>MENDMSSNQTLAEKKIPVSEVPSATLKMLTSQAEGVARPGGIFTKGDLINIKLYVKHSLELPFTLEGVKEYIGYNDIDIDGLKPAKMATLFKEIHDHALSWSGVESKVQQQSIDLENAGKQITLTGDEIISVIDQMPIIERVKNKLGDLTDKQLAEITYTNDDKEIAVELGNILESMKKDIKRQQENTQKVKTAVSDFKLKLIGGELSDGTIAQGLQPQISSKKKLMDDNNLSTTIKDLQSKIDEKNKEIDQFQKDYNKYVGLAFSGMVGGIISWAITGGIFGDKAEKARKQKNKLIDEVKDLQSQVKDKSALQTSVQNLSLSFAGIHTSMVDAEEALNHLDFMWNTMLTQITTSRDKFDDINDALKLTSFVIAFKQVIEPWRDVQGSAAQLIQTFDEALAEYKKLYH[2x]

α-Xenorhabdolysin is a PFT that has been first isolated from the bacterium Xenorhabdus nematophila. Xenorhabdolysins are also found in other entomopathogenic bacteria, such as Photorhabdus luminescens, and human pathogenic bacteria, such as Yersinia enterocolitica and Proteus mirabilis. They are composed of two subunits, namely XaxA (45 kDa) and XaxB (40 kDa) and are only active when the two components act together. Xenorhabdolysins, which were suggested to be binary toxins, perforate the membranes of erythrocytes, insect granulocytes and phagocytes and induce apoptosis. In contrast to previous predictions, XaxAB is therefore not a typical binary toxin, but rather a bi-component α-PFT.

XaxA crystallized in orthorhombic space group P212121 with a unit cell dimension of 67 × 90 × 153 Å and two molecules per asymmetric unit (AU). Phases were determined using the anomalous sulfur signal of the merged datasets and HKL2MAP, the graphical interface for SHELX C/D/E. The obtained phases combined with the given sequence and a few placed α-helices in the density with COOT were sufficient enough for phenix autobuild to almost completely build the structure of XaxA. Interestingly, XaxA contains two large loops connecting the helices, a big hook-shaped loop (lp1, aa 136–169) between helices αB and αC at the top of the tail domain and an additional loop (lp2, aa 202–215) dividing helix αC. In XaxA, the tip of the coiled-coil, predicted as hydrophobic transmembrane region is not resolved in our crystal structure, however, secondary structure predictions for this region suggest a continuation of the coiled-coil. Interestingly, in the case of XaxB the tongue is formed by an amphipathic helix, while XaxA does not contain such motif. Comparing the structure of XaxA with that of its pore conformation (see below) suggests that XaxA is already in its extended conformation as soluble monomer. The neck and head domains of XaxA are also arranged similarly to the crystal structure, however, the coiled-coil is twisted by 15 Å and interacts with helices αB and αC of the adjacent XaxB. XaxA alone has the tendency to form small aggregates by interacting with its head domain. Since the short hydrophobic region of the head domain resides inside the membrane in the pore complex, we believe that the clustering of XaxA monomers is caused by mild hydrophobic interactions of these regions. Interestingly, the protein was not incorporated into the liposomes and no larger structures could be observed on the vesicles. This indicates that albeit the hydrophobic tip of the head domain, XaxA cannot spontaneously insert blank membranes in vitro. Importantly, YaxA does not contain the hook-shaped loop (lp1), which is a prominent feature of XaxA.> MNTVRSEKDSMGAIDVPADKLWGAQTQRSLEHFRISTEKMPTSLIHALALTKRAAAKVNEDLGLLSEEKASAIRQAADEVLAGQHDDEFPLAIWQTGSGTQSNMNMNEVLANRASELLGGVRGMEAKVHPNDDVNKSQSSNDVFPTAMHVAALLALRKQLIPQLKTLTQTLNEKSRAFADIVKIGRTHLQDATPLTLGQEISGWVAMLEHNLKHIEYSLPHVAELALGGTAVGTGLNTHPEYARRVADELAVITCAP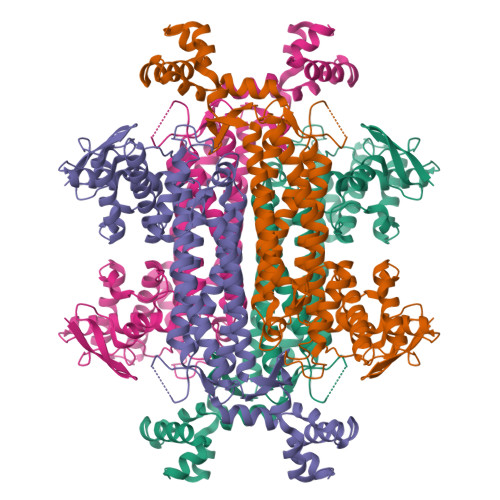FVTAPNKFEALATCDALVQAHGALKGLAASLMKIANDVRWLASGPRCGIGEISIPENEPGSSIMPGKVNPTQCEALTMLCCQVMGNDVAINMGGASGNFELNVFRPMVIHNFLQSVRLLADGMESFNKHCAVGIEPNRERINQLLNESLMLVTALNTHIGYDKAAEIAKKAHKEGLTLKAAALALGYLSEAEFDSWVRPEQMVGSMKAGRHHHHH> PGECSVNVIPKKNLDKAKFFSGTWYETHYLDMDPQATEKFCFSFAPRESGGTVKEALYHFNVDSKVSFYNTGTGPLESNGAKYTAKFNTVDKKGKEIKPADEKYSYTVTVIEAAKQSALIHICLQEDGKDIGDLYSVLNRNKNALPNKKIKKALNKVSLVLTKFVVTKDLDCKYDDKFLSSW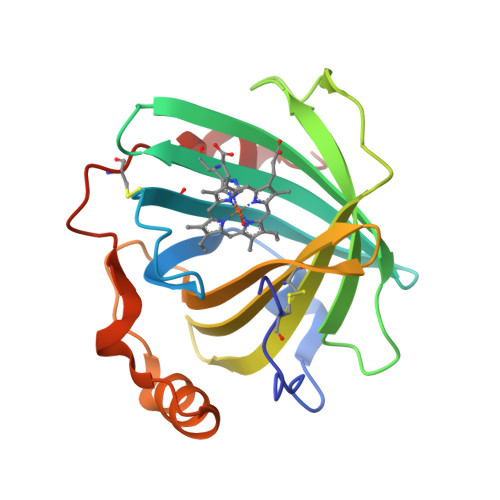QK ATP13A2, which is mutated in juvenile-onset Parkinson’s disease and autosomal recessive spastic paraplegia 78, is a transporter with a critical role in balancing the polyamine concentration between the lysosome and the cytosol. The overall structure of hATP13A2 has a canonical P-type ATPase architecture, with the cytosolic A domain linking to TM1 and TM2 domains, and the N and P domains sitting on the TM4 and TM5. The P-type ATPases transport substrates by coupling ATP hydrolysis with protein phosphorylation states and adopting a series of intermediate states, consisting of E1, E1-ATP, E1P-ADP, E1P, E2P, E2-Pi, and E2, in a process known as the Post-Albers reaction. Here, we report seven cryo-EM structures of hATP13A2 in six intermediate states, importantly including the putative E2 and E1-like states, thereby providing a nearly complete atomic-level conformational cycle spanning the Post-Albers reaction process.

In the map obtained after incubation with AMP-PCP (an ATP analog), a blob of density was clearly visualized near the KGSPE motif in the N-domain, suggesting the conformation of hATP13A2 was successfully trapped in the E1-ATP state. The ATP analog tethers together the N, P, and A domains of hATP13A2 in the E1-ATP state. During the transition from the E1-like to E1-ATP state, the A domain, P-domain, and N-domain of hATP13A2 are tightly tethered together by ATP to form a catalytic center for ATP hydrolysis and aspartic acid phosphorylation. Distinct from the E2P map, the E1-ATP map has no corresponding SPM density near Site1. The further structural comparison suggests that Site1 in the E1-ATP state is covered by three hydrophobic residues—W251, Y256, and F963—which may sterically hinder the binding of polyamine substrates. The first conformational change within the TM regions involves Site1, which is closed in the E1-ATP state, open in the E2P state, and closed in the putative E2 state, indicating a gate function of the entrance site during substrate recruitment. Adjustment of the inward-opening cavity was induced by the separation of TM2 and TM4b, which formed angles of ~30° and 37° in the E1-ATP and E2-Pi states, respectively.

> MSADSSPLVGSTPTGYGTLTIGTSIDPLSSSVSSVRLSGYCGSPWRVIGYHVVVWMMAGIPLLLFRWKPLWGVRLRLRPCNLAHAETLVIEIRDKEDSSWQLFTVQVQTEAIGEGSLEPSPQSQAEDGRSQAAVGAVPEGAWKDTAQLHKSEEAVSVGQKRVLRYYLFQGQRYIWIETQQAFYQVSLLDHGRSCDDVHRSRHGLSLQDQMVRKAIYGPNVISIPVKSYPQLLVDEALNPYYGFQAFSIALWLADHYYWYALCIFLISSISICLSLYKTRKQSQTLRDMVKLSMRVCVCRPGGEEEWVDSSELVPGDCLVLPQEGGLMPCDAALVAGECMVNESSLTGESIPVLKTALPEGLGPYCAETHRRHTLFCGTLILQARAYVGPHVLAVVTRTGFCTAKGGLVSSILHPRPINFKFYKHSMKFVAALSVLALLGTIYSIFILYRNRVPLNEIVIRALDLVTVVVPPALPAAMTVCTLYAQSRLRRQGIFCIHPLRINLGGKLQLVCFDKTGTLTEDGLDVMGVVPLKGQAFLPLVPEPRRLPVGPLLRALATCHALSRLQDTPVGDPMDLKMVESTGWVLEEEPAADSAFGTQVLAVMRPPLWEPQLQAMEEPPVPVSVLHRFPFSSALQRMSVVVAWPGATQPEAYVKGSPELVAGLCNPETVPTDFAQMLQSYTAAGYRVVALASKPLPTVPSLEAAQQLTRDTVEGDLSLLGLLVMRNLLKPQTTPVIQALRRTRIRAVMVTGDNLQTAVTVARGCGMVAPQEHLIIVHATHPERGQPASLEFLPMESPTAVNGVKDPDQAASYTVEPDPRSRHLALSGPTFGIIVKHFPKLLPKVLVQGTVFARMAPEQKTELVCELQKLQYCVGMCGDGANDCGALKAADVGISLSQAEASVVSPFTSSMASIECVPMVIREGRCSLDTSFSVFKYMALYSLTQFISVLILYTINTNLGDLQFLAIDLVITTTVAVLMSRTGPALVLGRVRPPGALLSVPVLSSLLLQMVLVTGVQLGGYFLTLAQPWFVPLNRTVAAPDNLPNYENTVVFSLSSFQYLILAAAVSKGAPFRRPLYTNVPFLVALALLSSVLVGLVLVPGLLQGPLALRNITDTGFKLLLLGLVTLNFVGAFMLESVLDQCLPACLRRLRPKRASKKRFKQLERELAEQPWPPLPAGPLR(4S)-2-tert-butylimidazo[1,2-a]pyrimidine 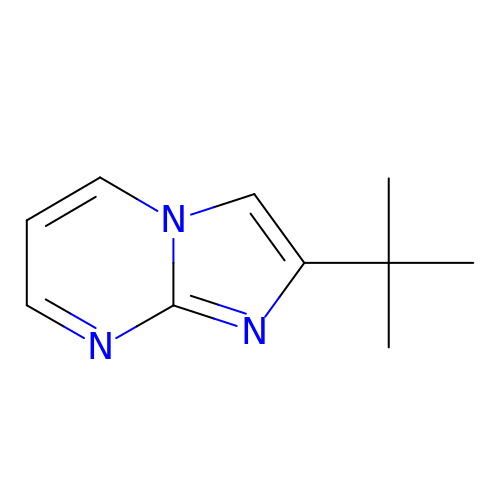| C10 H13 N3 | QCKNMBVCXLZFHY-UHFFFAOYSA-N4-METHOXYBENZOIC 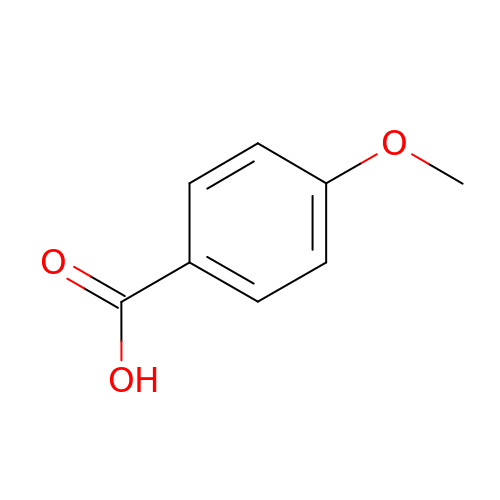ACID | C8 H8 O3 | ZEYHEAKUIGZSGI-UHFFFAOYSA-N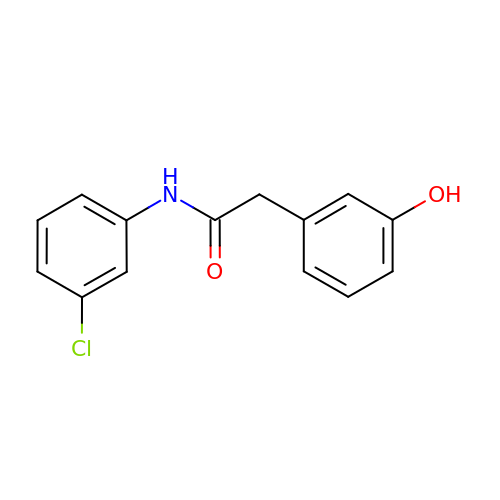N-(3-chlorophenyl)-2-(3-hydroxyphenyl)acetamide | C14 H12 Cl N O2 | SGQPJUCTSXTRQV-UHFFFAOYSA-N> KTDEKQLIIDAGQKRFGAVSCNVCGMLYTASNPEDETQHLLFHNQFISAVKYVGWKKERILAEYPDGRIIMVLPEDPKYALKKVDEIREMVDNDLGFQQAPLMCYSRTKTLLFISNDKKVVGCLIAEHIQWGYRVIEEKLPVIRSEEEKVRFERQKAWCCSTLPEPAICGISRIWVFSMMRRKKIASRMIECLRSNFIYGSYLSKEEIA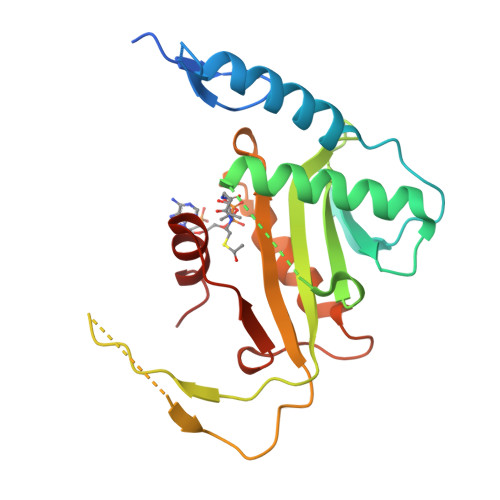FSDPTPDGKLFATQYCGT>[2x]ASDDNVFQPVDQLPEDLIPSSIQVLKFSGKYLKLEQDKAYFDWPGFKTAIDNYTGEDLSFDKYDQSTINQQSQEVGAMVDKIAKFLHDAFAAVVDLSKLAAIILNT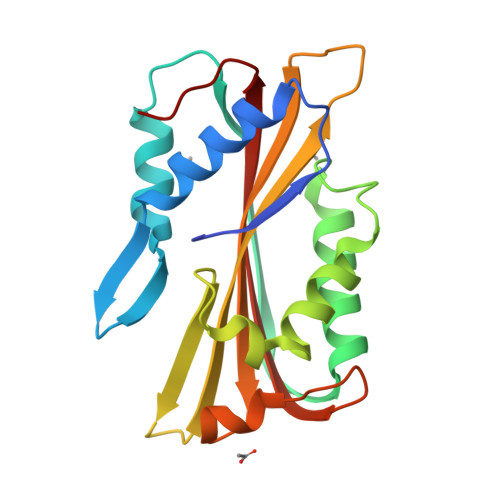FTNLEEESSSGFLQFNTNNVKKNSSWEYRVLFSVPFGDNAPSYFYSLVTTILITADIEEKTGWWGLTSSTKKNFAVQIDALELVVKKGFKAPN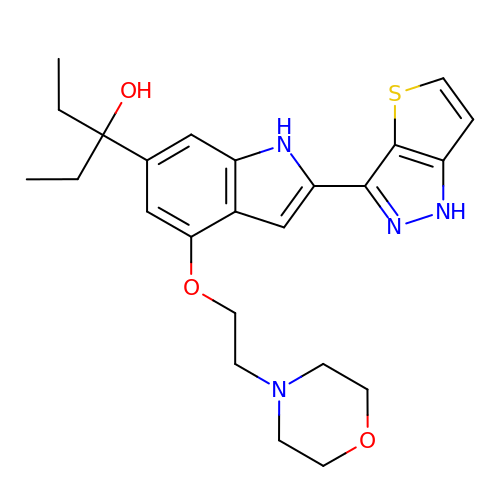3-[4-(2-morpholin-4-ylethoxy)-2-(1~{H}-thieno[3,2-c]pyrazol-3-yl)-1~{H}-indol-6-yl]pentan-3-ol | C24 H30 N4 O3 S | PVCKRSKEOOWVMP-UHFFFAOYSA-N>AYGIGLDITELKRIASMAGRQKRFAERILTRSELDQYYELSEARKNEFLAGRFAAKEAFSKAFGTGIGRQLSFQDIEIRKDQNGKPYIICTKLSQAAVHVSITHTKEYAAAQVVIERLSS[3x];>[3x]GPLGSADTLERVTKIIVDRLGVDEADVKLEASFKEDLGADXLDVVELVMELEDE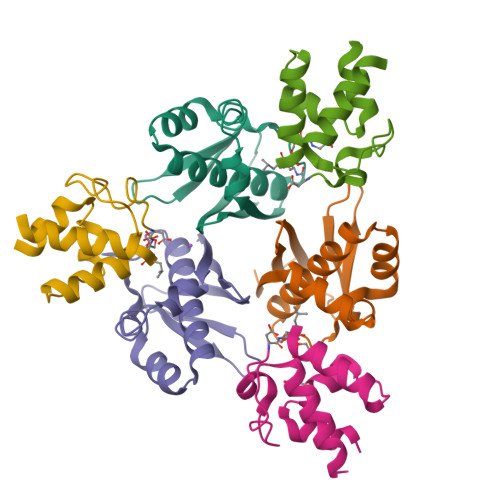FDMEISDEDAEKIATVGDAVNYIQNQQ>SEKYDGEWNEGRMQGWGKYFYADGGVYEGEWVDGRMHGRGTYVFPNGNKYEGEWVEDRKDGYGILLYTNGERYEGYWHLDKAHGKGTLTFLQGDRYVGEWHYGKKHGHGVLSYSNGDTYDGEWRDDDAWGYGVLQYANGCRYEGEWAEDRRHGKGLLVLPDGSSYEGSFAHGKKDGPGKIILKDGSMYIGTWKDGVIVGQGEFRLSENCDLSNPDY[2x]

High-resolution crystal structures and biophysical analyses of a truncated form of the TbMORN1 protein and its homologues from the parasites Toxoplasma gondii (TgMORN1) and Plasmodium falciparum (PfMORN1) enabled, for the first time, a structure-based definition of the MORN repeat. All three structures are antiparallel dimers joined via their C-termini, and, when possessed of the correct key residues, can adopt extended or V-shaped quaternary structures. The crystal structures confirmed that each 23-amino acid MORN repeat is composed of a β-hairpin followed by a 6-residue loop that connects to the next MORN repeat. The structural studies presented here make a case that one conserved function of MORN repeats is in homotypic interactions and possibly also in higher-order assembly.

The structures of TgMORN1(7–15) and both P21 and C2 crystal forms of TbMORN1(7–15) were subsequently determined to 2.90, 2.35 and 2.53 Å resolution, respectively, with the PfMORN1(7–15) structure used as a search model for the molecular replacement. TbMORN1(7–15) formed an extended antiparallel dimer in both crystal lattices, while TgMORN1(7–15) adopted this architecture in one crystal form. The two subunits in the TbMORN1(7–15) C2 crystal form and the TgMORN1(7–15) dimer make a rather straight assembly, while in the P21 form they display a bend of about 30°, leading to a rod-shaped particle appearance. The extended dimer interface is built from residues in MORN repeats 12–15, which connect the two subunits in an antiparallel, tail-to-tail orientation. The tightest overlap between the two subunits occurs through MORN repeats 14 and 15. A series of hydrophobic and aromatic π-stacking interactions between residues from repeats 14 and 15, together with hydrogen bonds across the edges, stabilise the dimer. Furthermore, the very negatively-charged C-terminal region of one TbMORN1 subunit forms an arch above the positively-charged platform contributed by Lys316 and Arg293. In the P21 and C2 TbMORN1(7–15) crystal forms, the dimer interfaces occupy surface areas of 747 Å2 and 966 Å2, respectively. Calculations of gain in solvation free energy (ΔiG) upon dimer formation for TbMORN1(7–15) C2 and P21 performed with the PDBePISA package yielded values of -20.1 kcal/mol and -11.3 kcal/mol, respectively, with corresponding p-values of interface specificity 0.01 and 0.08. ΔiG values lower than -10 to -15 kcal/mol and p-values lower than 0.5 are significant for stable protein dimers, indicating highly specific dimerisation interfaces. In the C2 crystal form, the dimer is additionally stabilised by two disulphide bridges formed between Cys351 at the C-terminus of repeat 15 and Cys282 from the β-hairpin loop of repeat 12.> KKGRHGAANDN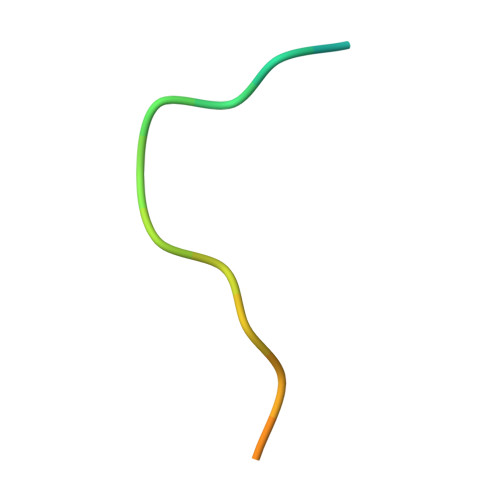FAEEFAVAA Human ATP:cob(I)alamin adenosyltransferase (ATR) is a mitochondrial enzyme that catalyzes an adenosyl transfer to cob(I)alamin, synthesizing 5′-deoxyadenosylcobalamin (AdoCbl) or coenzyme B12. ATR is also a chaperone that escorts AdoCbl, transferring it to methylmalonyl-CoA mutase, which is important in propionate metabolism. Mutations in ATR lead to methylmalonic aciduria type B, an inborn error of B12 metabolism. Human ATR is a homotrimer with active sites that are located at the subunit interfaces.

To gain structural insights into how the mutations impact AdoCbl binding, R190C and E193K ATR were cocrystallized with AdoCbl and PPPi, and the structures were solved by molecular replacement. Electron density that could be modeled as AdoCbl but not PPPi was present in the 1.8 Å structure of R190C and 2.2 Å structure of E193K ATR·AdoCbl. Both had four identical chains per asymmetric unit with an occupancy of one AdoCbl per monomer. Structural overlays revealed Cα RMSD values of 1.6 Å and 1 Å for WT ATR·ATP versus R190C·AdoCbl and E193K·AdoCbl, respectively, indicating that the mutations do not induce major conformational changes in the overall structure. AdoCbl was bound in the base-off conformation with Phe-170 positioned at a distance of 3.6 Å from the cobalt atom. An overlay of the WT and E193K ATR structures revealed only subtle differences in the orientation of the deoxyadenosyl moiety. Indeed, structural changes that might explain the profoundly lower affinity of E193K ATR for AdoCbl (±PPPi) were not obvious in the crystal structure. It is likely that the E193K mutation impacts protein dynamics by destabilizing the β−hairpin roof and, therefore, the active site architecture. Although Glu-193 makes a single electrostatic interaction with the amino group of the adenine moiety, it plays a role in stabilizing the β-hairpin roof over the active site via its interaction with Lys-78. Hence, the E193K mutation is predicted to primarily impair the chaperone function of ATR by weakening its affinity for PPPi and AdoCbl in the ternary product complex.

>MPKIYTKTGDKGFSSTFTGERRPKDDQVFEAVGTTDELSSAIGFALELVTEKGHTFAEELQKIQCTLQDVGSALATPCSSAREAHLKYTTFKAGPILELEQWIDKYTSQLPPLTAFILPSGGKISSALHFCRAVCRRAKRRVVPLVQMGETDANVAKFLNRLSDYLFTLARYAAMKEGNQEKIYMKNDPSAESEGL[4x]> MSSSPCDQLQSFADGDLPPMEAQAFGQHLADCEKCQVELTRLLQLDQLGRGYIERHGPVDIPWHALPRNRWMAGGFALASMVAVAFILLGTLRPQAPRALPELWAQPQRTLEARVTYLAADRYRRPPQVMMGGAAARSGPNRSLALLSELEKRGDLHQLAVAYLATGVPEPSSAKAILEGMRSDLRWQSADVLCDLGVAHYVASKPLDAARATEELREALRLFDTVLAMQPGHVQALWNRSLVYRDLGLPLSAMKDLTEFEHRETDEGWRSEARDRRARLSSTLRRKERWLAADQTGADLINRGAQELARALTFVDVPLLRRDFYHAVRARTSSTDVLALLPLAERLDASVGSGTVLADYVHQVAARDFSRRAPLAEQYARLISGRIPESEQDALLQRFLTSDETDLALGALAHVMQRLPAYASELVRRTQHDEDPWFRVLGLQAQAMLERQQEHYKEALAPLEQALDICRRERLVYRCIFIENDLSHVKSWLFRVNAAAQHARDGLALARPNQWDLEGVMLQALGNVARQAADVTLGRAYYGEALLMAEGDKWSTRN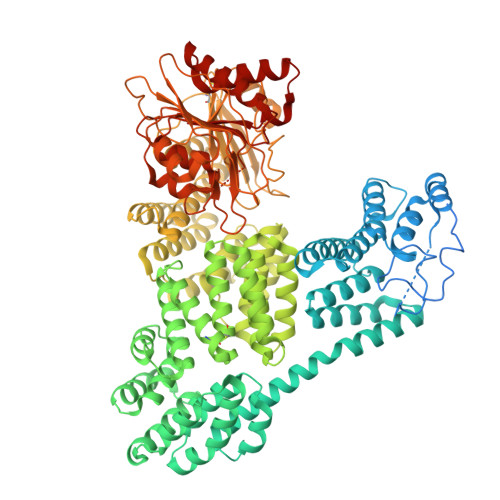IHQNLAHLAIWALELDEARASLDRAMDTGLPLTQHGVAALVDVARTRRSPRDALMVEQALAREPGNTPGQRAYAKFLHGRILVEVDPARGRMLLDEAIRQAEALPLDDVSAAHARAYSYTSLIFADADTGDFIAALARFGAELGFETPARCVLGLTADTERSLLVARGAQGQLLSAYVPLRSSRFEAASMEGAVPPEMLAALQACTLVDVLARPPLQGRSGLLPPGIAWRYRTRAAAPPPPAGPGTHLVVNEVRYSEERNEVPLQWLPRTAPGAEARFLRDLAATPTQVLEAISTATEIDLATHGKVDPDSNFAYLLLAPGADGRDTLFEDSIRASQLTGAPLVVLAACEGGRPNAALHRAGSLPSAFLAAGARAVLAATHPIPDLDSSAFFGAVRDRVLAGASLAVAVRDERLQWLSAGGDSEWVNAVLVFE>[2x]QAKHKQRKRLKSSCKRHPLYVDFSDVGWNDWIVAPPGYHAFYCHGECPFPLADHLNSTNHAIVQ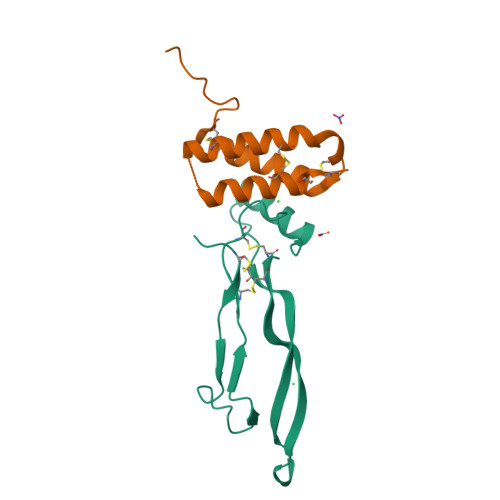TLVNSVNSKIPKACCVPTELSAISMLYLDENEKVVLKNYQDMVVEGCGCR;>[2x]ETSQCKILRCNAEYVSSTLSLRGGGSSGALRGGGGGGRGGGVGSGGLCRALRSYALCTRRTARTCRGDLAFHSAVHGIEDLMIQHNCSRQGPTAPPPPRGPALPGAGSGLPAPGTKHHHHHH>GIDPFTGYQLSATLKGHDQDVRDVVAVDDSKVASVSRDGTVRLWSKDDQWLGTVVYTGQGFLNSVCYDSEKELLLFGGKDTMINGVPLFATSGEDPLYTLIGHQGNVCSLSFQDGVVISGSWDKTAKVWKEGSLVYNLQAHNASVWDAKVVSFSENKFLTASADKTIKLWQNDKVIKTFSGIHNDVVRHLAVVDDGHFISCSNDGLIKLVDMHTGDVLRTYEGHESFVYCIKLLPNGDIVSCGEDRTVRIWSKENGSLKQVITLPAISIWSVDCMSNGDIIVGSSDN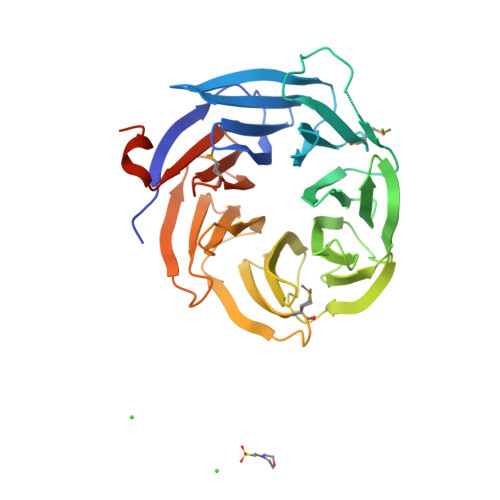LVRIFSQEKSRWASEDEIKGELRSGC[2x]Sizzled (Szl) is both a secreted frizzled related protein (sFRP) and a naturally occurring inhibitor of the zinc metalloproteinase bone morphogenetic protein-1 (BMP-1), a key regulator of extracellular matrix assembly and growth factor activation. In most vertebrates (with the exception of mammals) this gradient is finely tuned by the presence of the protein Sizzled (Szl) which is a potent and specific inhibitor of BTPs (Ki = 1.5 nM). Bone morphogenetic protein-1 (BMP-1, EC 3.4.24.19) is a secreted multidomain Zn-metallopeptidase of the astacin M12A subfamily which plays a key role in extracellular matrix (ECM) deposition, growth factor activation and the generation of animal form. As a member of the BMP-1/tolloid-like family (BTPs), BMP-1 controls ECM deposition by site-specific proteolysis of procollagens, proteoglycans, prolysyl oxidases and other matrix proteins; BTPs also control growth factor activity, particularly members of the TGF-β superfamily, by proteolytic cleavage of precursor forms or growth factor antagonists.

Here we present a new crystal structure for Szl which differs from that previously reported by a large scale (90°) hinge rotation between its cysteine-rich and netrin-like domains. Crystals from native and selenomethionine-labelled Szl belonged to space groups P212121 and P21 and diffracted X-rays to 1.95 and 3.32 Å, respectively. The crystal structure was determined by combining SAD phasing using the Szl-SeMet data with a partial molecular replacement model from the high-resolution native data (1.95 Å) and refinement to the same resolution. The final refined model includes two chains (A and B) containing 235 and 241 amino acids, respectively. The structural fold of Szl is stabilized by eight disulphide bonds (seven intra-domain formed by cysteines 27–90, 37–83, 74–109, 98–136, 102–126, 159–231, 176–281 and one inter-domain formed by cysteines 115–156). No electron density was observed for the linker (residues 138–150) connecting the CRD to the NTR domain, probably due to high flexibility. In contrast, the NTR domain displays mixed β-α-β topology, consisting of seven β-strands (β3–β9), flanked by helices α5–α8. Instead, there was a rotation about the long axis of one domain with respect to the other of approximately 90°, pivoting around the inter-domain disulphide bridge. Despite its interdomain disulphide bridge, not present in other SFRPs except Crescent, Szl has remarkable freedom of movement about its CRD and NTR domains.

>[2x]ETGFDIGLSTKCVTIPTEMAMCNDVGYSEMRLPNLMGHTNMAEVVPKSAEWQNLLQTGCHPYARTFLCSLFAPVCLDTFIQPCRSMCVAVRDSCAPVLACHGHSWPESLDCDRFPAGEDMCLDTLSKEYQYSYKELPKPSCQGCPLIEEFFSHKTVLEAFCDNNFAVKVKLAKKKSASGLYEYETEGPVEFIKQGLLLPYDTRTMIEQWLLINENCAQKLIRTRPTVYVIAGDIHHGKVKVNRIFHWQKKDSQLTLATRRWRHHKCGTKHHHHHH Matrix protein (MA), p15 in FIV or EIAV and p17 in HIV or SIV, is the N-terminal subunit of the retroviral Gag polyprotein. During the viral replication cycle, the FIV p15 matrix protein oligomerizes to form a closed matrix that underlies the lipidic envelope of the virion. In FIV, HIV or SIV, the N-terminal domain of Gag undergoes a co-translational covalent modification of the MA N-terminus with a myristoyl group. This myristoylation, together with a highly basic patch of amino acid residues located at the N-terminus of the MA, directs the Gag polyprotein to the plasma membrane (PM), mediating the association between Gag and the inner leaflet of the PM lipid bilayer, where Gag forms a hexagonal network. The structure consists of five α-helices (numbered h1 to h5 following the HIV convention), which give rise to the close packing of adjacent helices typical for retroviral matrix proteins.

FIV full-length p15 protein at 6 mg/ml in MES buffer pH 6 crystallizes in the presence of sodium acetate pH 4.6 and PEG in the space group P21212 with one molecule in the asymmetric unit. Synchrotron data were collected to 2 Å resolution. The three amino-terminal residues (Gly4-Gln5-Gly6) and the twenty carboxy-terminal residues (Met113 to Gln133) are mainly unstructured and extended. Despite its intrinsic flexibility, the C-terminal end (Met113 to Gln133) is clearly observed in the electron density map because of the stabilizing crystal contacts of the C-terminal residues 130 to 132 with the complementary monomer. An analysis of the electrostatic potential of FIV full-length p15 revealed a highly basic platform, with helix h1 having amphipathic character (residues Arg7 to Cys16). As with HIV, a hydrophobic cavity formed by the side chains of helices h1 to h4 is observed in the FIV p15 protein. The C-terminal end of FIV p15 is mainly unstructured and extended, whereas a long helix h5 is observed in HIV p17, and a short β-hairpin is reported in SIV MA. The first interface (interface 1) implicates the conserved residue Trp37, localized at the center of helix h2 and the C-terminal end of a contacting p15 monomer (Gly130 to Pro132). Of interest, the indol group of Trp37 makes extensive contacts with the Pro131 of the complementary molecule via hydrophobic stacking. Unlike SIV, HIV and EIAV MA, FIV p15 appears monomeric in the crystal, although it is dimeric in the protein solution used for crystallization.

> MGNGQGRDWKMAIKRCSNVAVGVGGKSKKFGEGNFRWAIRMANVSTGREPGDIPETLDQLRLVICDLQERREKFGSSKEIDMAIVTLKVFAVAGLLNMTVSTAAAAENMYSQMGLDTRPSMKEAGGKEEGPPQAYLVPRGSLEHHHHHH>[2x]GPMLADLDHFGKNYKHDEEAQRNQKPWMLTWPQIKLVLLAGVGFFLDAYDLFIINQVAPMLAQVYFPKTGLPAQRQDLMKAAANIGCVVGQVMFGVLGDSFGRKFVYGKELILIIVATIFQMSAPSHWDGNRVLTWITICRVFLGIGIGGDYPMSATVVSDRANIHRRGTLLCFIFANQGWGSFVGSLVTIVTISGFKHRLKSGHTHDVDKAWRILIGLSLIPAFGTLYQRLTLPESRKFELTRDAASSSTVAIDKKDHDATHEVKDAPESEKSSPKVTPADAIDDDRHGVIASKKAHWQEFVAYFSTWNHFRNLLGSMLGWFLVDI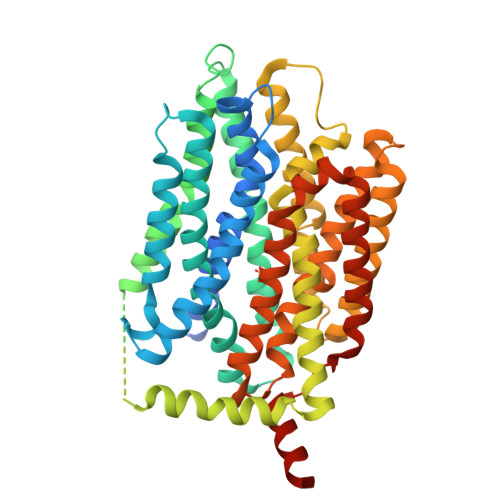AFFGINLNQSVVLAQIGFAGKTGDVYDKLFQLATGNIIVTALGFLPGYYFTLFLIDIVGRKKLQFMGFIMSGLFLAILAGEIDHIGKGPLLACFTFMQFFFNFGANTTTFIVAAELFPTRIRASAHGISAAAGKCGAILSSLVFNQLKAKIGTSAVLWIFFSTCILGFISTFLIDETMGVDPDEKDLEERRARGEIPGGLVPR> MAFSELLDLVGGLGRFQVLQTMALMVSIMWLCTQSMLENFSAAVPSHRCWAPLLDNSTAQASILGSLSPEALLAISIPPGPNQRPHQCRRFRQPQWQLLDPNATATSWSEADTEPCVDGWVYDRSIFTSTIVAKWNLVCDSHALKPMAQSIYLAGILVGAAACGPASDRFGRRLVLTWSYLQMAVMGTAAAFAPAFPVYCLFRFLLAFAVAGVMMNTGTLLMEWTAARARPLVMTLNSLGFSFGHGLTAAVAYGVRDWTLLQLVVSVPFFLCFLYSWWLAESARWLLTTGRLDWGLQELWRVAAINGKGAVQDTLTPEVLLSAMREELSMGQPPASLGTLLRMPGLRFRTCISTLCWFAFGFTFFGLALDLQALGSNIFLLQMFIGVVDIPAKMGALLLLSHLGRRPTLAASLLLAGLCILANTLVPHEMGALRSALAVLGLGGVGAAFTCITIYSSELFPTVLRMTAVGLGQMAARGGAILGPLVRLLGVHGPWLPLLVYGTVPVLSGLAALLLPETQSLPLPDTIQDVQNQAVKKATHGTLGNSVLKSTQF

The human urate transporter 1 (hURAT1) plays a critical role in urate homeostasis by facilitating urate reabsorption in the renal proximal tubule, making it a key target for gout therapy. The human urate transporter 1 (URAT1) is a crucial member of the SLC22A subfamily, which includes both organic anion transporters (OATs) and organic cation transporters (OCTs). The overall architecture of URAT1 comprises three distinct regions: the transmembrane domain (TMD), the extracellular domain (ECD), and a predicted intracellular helical (ICH) bundle, which was not resolved in our structures. The TMD of URAT1 displays a characteristic Major Facilitator Superfamily (MFS) topology, consisting of 12 transmembrane helices arranged in two pseudo-symmetric halves: the N-terminal domain (NTD, TM1–TM6) and the C-terminal domain (CTD, TM7–TM12).

The 3.3 Å resolution structure of URAT1 in complex with urate revealed critical details about the substrate binding site. The density maps clearly showed urate bound within a pocket formed by residues from transmembrane helices TM5, TM7, TM8, and TM10. The urate molecule primarily engages in π-stacking interactions with phenylalanine residues F241, F360, F364, F365, and F449. Additionally, a polar interaction between urate and K393 further stabilizes the binding, as evidenced by the substantial decrease in transport activity upon K393A mutation. Interestingly, we observed that S35 in TM1 forms a water-mediated hydrogen bond with urate. Alanine substitution of S35 also resulted in a notable reduction in the transport activity of URAT1, highlighting the importance of this interaction. While transporters like OAT1 typically employ a combination of phenylalanine and tyrosine residues to create their substrate-binding aromatic cages, URAT1 exclusively utilizes phenylalanine residues. This characteristic likely renders the binding pocket of URAT1 more hydrophobic than those of other transporters. Moreover, the binding pocket is relatively narrow, with an 8.2 Å separation between F241 and F449, compared to ~9.1 Å in rOAT1. These features impose stringent selection criteria based on substrate polarity and size, contributing to the high substrate specificity observed for URAT1.3-{3-[(pyridin-2-yl)methoxy]quinoxalin-2-yl}propanoic 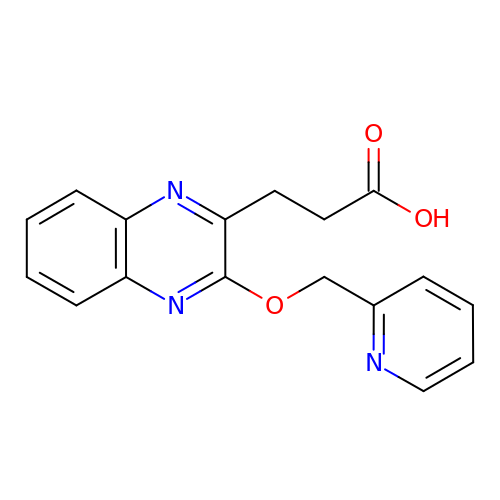acid | C17 H15 N3 O3 | TXJSUZJFIYIMRT-UHFFFAOYSA-N>[6x]PVVIKTEGPAWTPLEPKLITRLADTVRTKGLRSPITMAEVEALMSSPLLPHDVTNLMRVILGPAPYALWMDAWGVQLQTVIAAATRDPRHPANGQGRGERTNLNRLKGLADGMVGNPQGQAALLRPGELVAITASALQAFREVARLAEPAGPWADIMQGPSESFVDFANRLIKAVEGSDLPPSARAPVIIDCFRQKSQPDIQQLIRTAPSTLTTPGEIIKYVLDRQKTA

As the virus buds from the cell, the viral protease cleaves Gag into several fragments, including the capsid protein (CA) that then assembles into the mature capsid shell (core), rendering the virus particle infectious. The CA portion of all retroviral Gag proteins folds into two separate domains, the N-terminal domain (CANTD) and C-terminal domain (CACTD). In mature lattices, CANTD interactions form only intra-hexamer and intra-pentamer interfaces, while CACTD interactions are also involved in formation of inter-hexamer and inter-pentamer interfaces. Our results show that, like lentiviruses, RSV is sensitive to IP6 in vitro and in cells, where in the mature CA lattice IP6 binds in a pore formed in the center of the CANTD hexamer.

Further analysis of the different hexamers forming the mature CA lattice in polyhedral CLPs revealed that despite the deformability of the CA hexamer, local symmetries exist in the lattice. Aside from the C2-symmetric hexamers that are also observed in regular tubes (and are surrounded by only hexamers, Fig. 3b group V), a fraction of hexamers in the polyhedrons were surrounded by either two or three pentamers in a symmetrical manner and hence followed C2 symmetry and C3 symmetry, respectively. In contrast, the structures of the other two-symmetric hexamers highlight the structurally dominant influence of the pentamer, where it actively defines the conformation of its adjacent hexamers. Specifically, the two CA monomers facing a pentamer adopt an arrangement similar to those two CA monomers in the pentamer, causing an increased spatial separation between the CANTD’s of the hexamer. This observation was further confirmed via the structure determination of a small set of T = 3 icosahedral particles solved by single-particle cryo-EM. In T = 3 icosahedrons each hexamer is surrounded by three pentamers, which causes the described threefold-symmetric distortion of the CA hexamer. The similarity of the C3 hexamer from the T = 3 icosahedra (formed by CA) to the C3 hexamer from the polyhedrons (formed by CASPNC and IP6) suggests that the structural deviation from C6 symmetry is not due to the presence of either the IP6 molecule, nor the absence of the β-hairpin, nor the SPNC region.> SNADPYIAVVSKGFQHKFWVTVRDGAEAAAKQNGVKISFV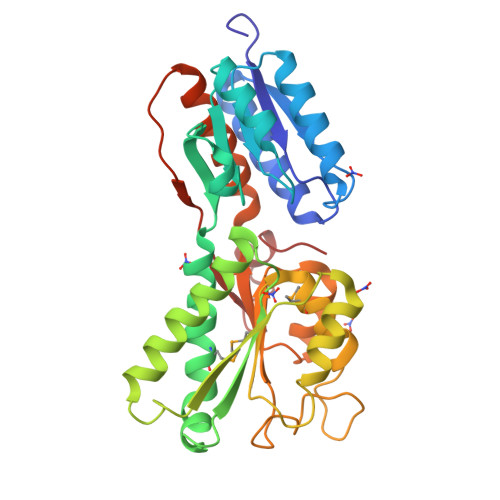GPETESDSKIQQDLLDSEINKNPDAIAFAAVTGDFTEQIKRIKEKNIPLIGFDSGILPDQAQGAVLATASTDNRAAAAIVADKMFEALKTRIAAFTSDNKAKIAVLQLDNSDTGIGRAEGFVKRFTELADGDAATAGKYALQVIVPTTQNEADIANEVNALRGKSVLGIYLSNEAMARGFLVVYKSAEAGAANTIVGDAQDGGDLVVMGFDSGKPQLDAIRNGIIQGSVTQDPYSIGFQAVTLAYKASKGESVSNIDTGAKWYDKTNIDDPEIAKLLYE(5-hydroxy-4-{[(1-hydroxy-2-oxo-1,2-dihydroquinolin-3-yl)amino]methyl}-6-methylpyridin-3-yl)methyl 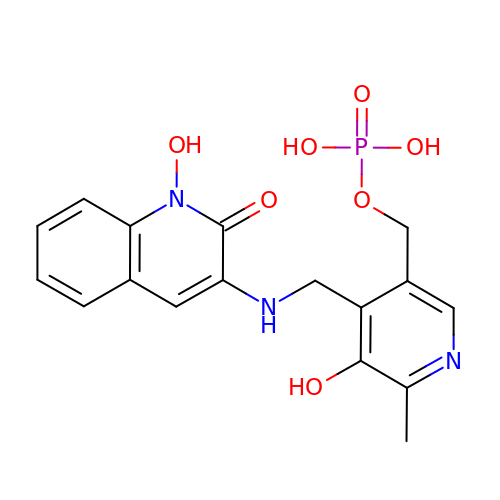dihydrogen phosphate | C17 H18 N3 O7 P | ZKPXUQQBRMXHLJ-UHFFFAOYSA-N>SGGSMLYVSNLPVGTSSSAIHALFSAYGNVKDIWMLSPDNSAIVSYESLSSAIVARDALHNRPVFENHGPVQVMLA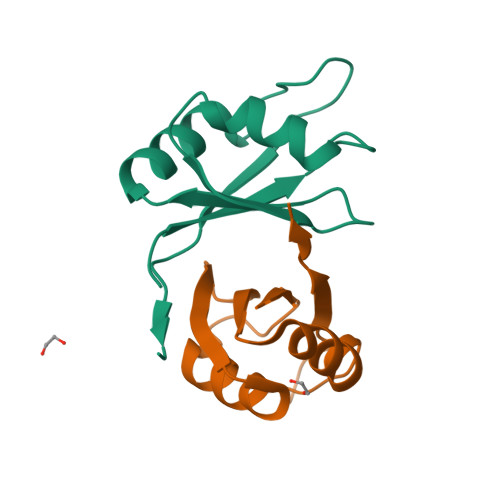KPSSNYE[4x]>RLTELREDIDAILEDPALEGAVSGVVVVDTATGEELYSRDGGEQLLPASNMKLFTAAAALEVLGADHSFGTEVAAESAPGRRGEVQDLYLVGRGDPTLSAEDLDAMAAEVAASGVRTVRGDLYADDTWFDSERLVDDWWPEDEPYAYSAQISALTVAHGERFDTGVTEVSVTPAAEGEPADVDLGAAEGYAELDNRAVTGAAGSANTLVIDRPVGTNTIAVTGSLPADAAPVTALRTVDEPAALAGHLFEEALESNGVTVKGDVGLGGVPADWQDAEVLADHTSAELSEILVPFMKFSNNGHAEMLVKSIGQETAGAGTWDAGLVGVEEALSGLGVDTAGLV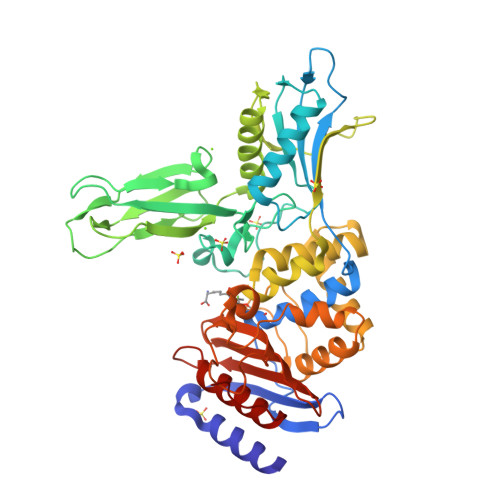LNDGSGLSRGNLVTADTVVDLLGQAGSAPWAQTWSASLPVAGESDPFVGGTLANRMRGTAAEGVVEAKTGTMSGVSALSGYVPGPEGELAFSIVNNGHSGPAPLAVQDAIAVRLAEYAGHQAPEG[4x]> MIRKKILMAAIPLFVISGADAAVSLDRTRAVFDGSEKSMTLDISNDNKQLPYLAQAWIENENQEKIITGPVIATPPVQ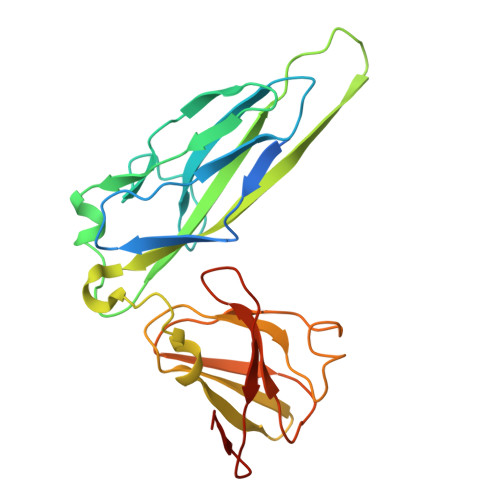RLEPGAKSMVRLSTTPDISKLPQDRESLFYFNLREIPPRSEKANVLQIALQTKIKLFYRPAAIKTRPNEVWQDQLILNKVSGGYRIENPTPYYVTVIGLGGSEKQAEEGEFETVMLSPRSEQTVKSANYNTPYLSYINDYGGRPVLSFICNGSRCSVKKEK>MAGPLSGLRVVELAGIGPGPHAAMILGDLGADVVRIDRPSSVDGISRDAMLRNRRIVTADLKSDQGLELALKLIAKADVLIEGYRPGVTERLGLGPEECAKVNDRLIYARMTGWGQTGPRSQQAGHDINYISLNGILHAIGRGDERPVPPLNLVGDFGGGSMFLLVGILAALWERQSSGKGQVVDAAMVDGSSVLIQMMWAMRATGMWTDTRGANMLDGGAPYYDTYECADGRYVAVGAIEPQFYAAMLAGLGLDAAELPPQNDRARWPELRALLTEAFASHDRDHWGAVFANSDACVTPVLAFGEVHNEPHIIERNTFYEAN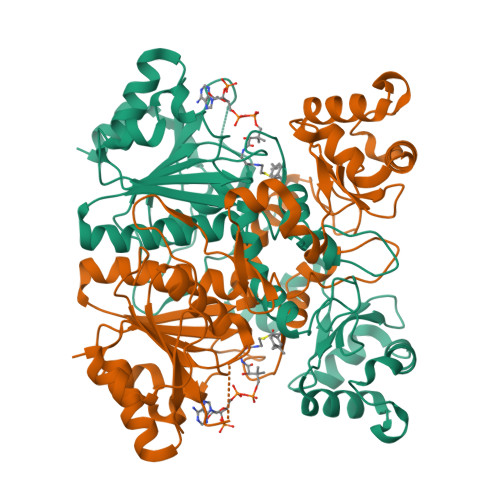GGWQPMPAPRFSRTASSQPRPPAATIDIEAVLTDWDGGSGC[12x]1-[5-({4-[3-chloro-5-(trifluoromethyl)phenyl]piperazin-1-yl}sulfonyl)-2,3-dihydro-1H-indol-1-yl]ethan-1-one | C21 H21 Cl F3 N3 O3 S | 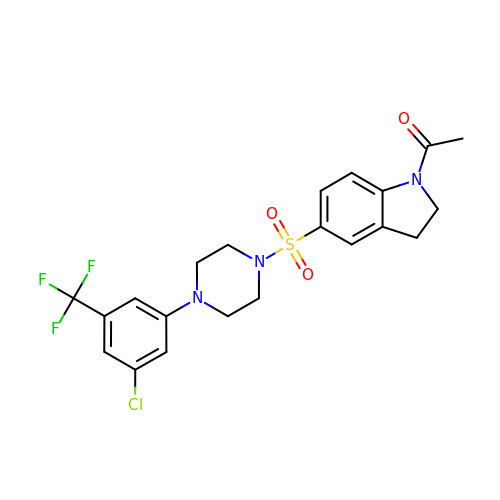PDEIRNVIXFZSSJ-UHFFFAOYSA-N>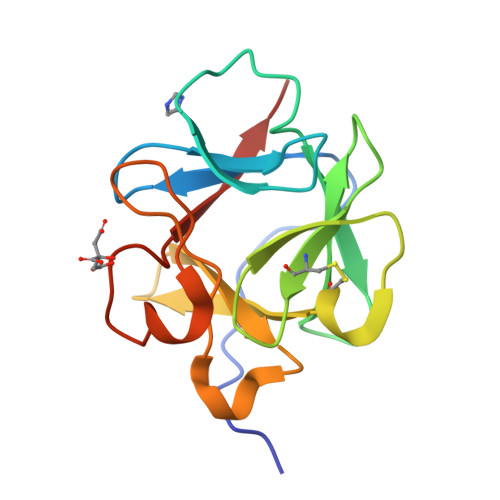[2x]MHHHHHHFNLPPGNYKKPKLLYSSNGGHFLRILPDGTVDGTRDRSDQHIQLQLSAESVGEVYIKSTETGQYLCMDTDGLLYGSQTPNEECLFLERLEENHYNTYISKKHAEKNWFVGLKKNGSAKRGPRTHYGQKAILFLALPVSSD> MELIKGQALFLELDKKDFLSLKNNDKNIPTFAHPKNQEKILAIFSLPYKNPPQNTKLIAFYKDKKEEIFIKTLEGNYKSEKLQVENKKIFPPKTIQERIAKELKEANAIYSSYTPKALFNGAFNIPLNSFITSDFGKARTFNEKVASYHSGTDFRAATGTPIYAANSGVVKIAKDRYFAGNSVVIDHGFGIYSQYYALSKIDVKVGQKIKKGELIGLSGASGRVSGPHLHFGILAGGKQVDPLDFVSKFNAIFQLEHHHHHH

We have described herein the reactions and the structure of Pgp3, a Csd protein of C. jejuni. This enzyme turns over the cell-wall peptidoglycan by both the d,d-endopeptidase and d,d-carboxypeptidase activities, as documented by mass spectrometric characterization of the requisite reactions with synthetic cell-wall fragments. The Pgp3 monomer is structurally divided into four regions: the N-terminal domain (NTD, residues 21–95), a flexible linker (residues 96–147), the LytM domain (residues 148–259), and the C-terminal helix (residues 260–273). The Pgp3 LytM domain contains a highly conserved tetrahedral Zn2+-ion-binding motif (H168xxxD172 and HxH249).

The structures are: (i) tartrate-bound wild type (WT) (open form), (ii) citrate-bound WT (two structures, closed form), (iii) H216A mutant (open form), (iv) H216A mutant with tartrate (closed form), (v) H247A mutant (open form), (vi) H247A mutant with pentapeptide 1, Ac-l-Ala1-γ-d-Glu2-mDAP3-d-Ala4-d-Ala5 (open form), and (vii) H247A mutant with crosslinked muramyl tetra-tri peptide 2, NAM-l-Ala1-γ-d-Glu2-mDAP3-d-Ala4-mDAP3-γ-d-Glu2-Ala1-NAM (open form). The amino acids His216 and His247 are strictly conserved for Wat-1 and Wat-2 coordination in the M23 metallopeptidase family, and for the core of the catalytic machinery. We decided to mutate His216 and His247 individually to alanine in order to abrogate the binding of tartrate or citrate at the active site and impair catalysis too. In the case of the H216A variant, tartrate was sometimes observed in the closed form crystal structure; hence, only the H247A variant was pursued further. Since crystals of Pgp3 contained one or three subunits in the asymmetric unit of WT and variants (H216A and H247A, both discussed later) depending on the space group, we analyzed the oligomeric states of the WT and variant Pgp3 in solution using size-exclusion chromatography with multi-angle light scattering (SEC-MALS) experiments. The molecular masses of the WT, H216A, and H247A variants were 28.4, 28.9, and 30.0 kDa, respectively, close to the theoretical molecular mass of the Pgp3 monomer (29.4 kDa). These results indicate that the likely functional state of Pgp3, as measured herein in solution, is monomeric.> MSEKRSLPMVDVKIDDEDTPQLEKKIKRQSIDHGVGSEPVSTIEIIPSDSFRKYNSQGFKAKDTDLMGTQLESTFEQELSQMEHDMADQEEHDLSSFERKKLPTDFDPSLYDISFQQIDAEQSVLNGIKDENTSTVVRFFGVTSEGHSVLCNVTGFKNYLYVPAPNSSDANDQEQINKFVHYLNETFDHAIDSIEVVSKQSIWGYSGDTKLPFWKIYVTYPHMVNKLRTAFERGHLSFNSWFSNGTTTYDNIAYTLRLMVDCGIVGMSWITLPKGKYSMIEPNNRVSSCQLEVSINYRNLIAHPAEGDWSHTAPLRIMSFSISCAGRIGVFPEPEYDPVIQIANVVSIAGAKKPFIRNVFTLNTCSPITGSMIFSHATEEEMLSNWRNFIIKVDPDVIIGYNTTNFDIPYLLNRAKALKVNDFPYFGRLKTVKQEIKESVFSSKAYGTRETKNVNIDGRLQLDLLQFIQREYKLRSYTLNAVSAHFLGEQKEDVHYSIISDLQNGDSETRRRLAVYCLKDAYLPLRLMEKLMALVNYTEMARVTGVPFSYLLARGQQIKVVSQLFRKCLEIDTVIPNMQSQASDDQYEGATVIEPIRGYYDVPIATLDFNSLYPSIMMAHNLCYTTLCNKATVERLNLKIDEDYVITPNGDYFVTTKRRRGILPIILDELISARKRAKKDLRDEKDPFKRDVLNGRQLALKISANSVYGFTGATVGKLPCLAISSSVTAYGRTMILKTKTAVQEKYCIKNGYKHDAVVVYGDTDSVMVKFGTTDLKEAMDLGTEAAKYVSTLFKHPINLEFEKAYFPYLLINKKRYAGLFWTNPDKFDKLDQKGLASVRRDSCSLVSIVMNKVLKKILIERNVDGALAFVRETINDILHNRVDISKLIISKTLAPNYTNPQPHAVLAERMKRREGVGPNVGDRVDYVIIGGNDKLYNRAEDPLFVLENNIQVDSRYYLTNQLQNPIISI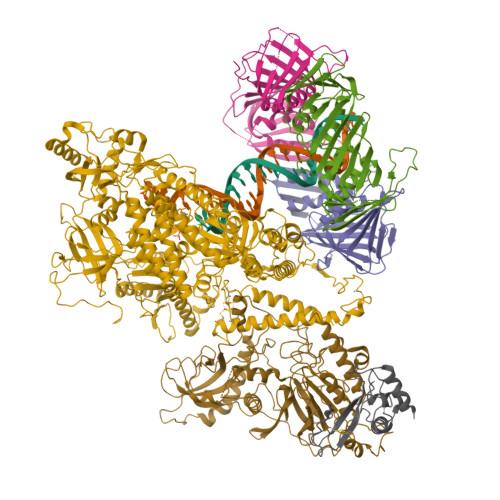VAPIIGDKQANGMFVVKSIKINTGSQKGGLMSFIKKVEACKSCKGPLRKGEGPLCSNCLARSGELYIKALYDVRDLEEKYSRLWTQCQRCAGNLHSEVLCSNKNCDIFYMRVKVKKELQEKVEQLSKW;> MDALLTKFNEDRSLQDENLSQPRTRVRIVDDNLYNKSNPFQLCYKKRDYGSQYYHIYQYRLKTFRERVLKECDKRWDAGFTLNGQLVLKKDKVLDIQGNQPCWCVGSIYCEMKYKPNVLDEVINDTYGAPDLTKSYTDKEGGSDEIMLEDESGRVLLVGDFIRSTPFITGVVVGILGMEAEAGTFQVLDICYPTPLPQNPFPAPIATCPTRGKIALVSGLNLNNTSPDRLLRLEILREFLMGRINNKIDDISLIGRLLICGNSVDFDIKSVNKDELMISLTEFSKFLHNILPSISVDIMPGTNDPSDKSLPQQPFHKSLFDKSLESYFNGSNKEILNLVTNPYEFSYNGVDVLAVSGKNINDICKYVIPSNDNGESENKVEEGESNDFKDDIEHRLDLMECTMKWQNIAPTAPDTLWCYPYTDKDPFVLDKWPHVYIVANQPYFGTRVVEIGGKNIKIISVPEFSSTGMIILLDLETLEAETVKIDI;> MDQKASYFINEKLFTEVKPVLFTDLIHHLKIGPSMAKKLMFDYYKQTTNAKYNCVVICCYKDQTIKIIHDLSNIPQQDSIIDCFIYAFNPMDSFIPYYDIIDQKDCLTIKNSYELKVSESSKIIERTKTLEEKSKPLVRPTARSKTTPEETTGRKSKSKDMGLRSTALLAKMKKDRDDKETSRQNELRKRKEENLQKINKQNPEREAQMKELNNLFVEDDLDTEEVNGGSKPNSPKETDSNDKDKNNDDLEDLLETTAEDSLMDVPKIQQTKPSETEHSKEPKSEEEPSSFIDEDGYIVTKRPATSTPPRKPSPVVKRALSSSKKQETPSSNKRLKKQGTLESFFKRKAK;>MLEAKFEEASLFKRIIDGFKDCVQLVNFQCKEDGIIAQAVDDSRVLLVSLEIGVEAFQEYRCDHPVTLGMDLTSLSKILRCGNNTDTLTLIADNTPDSIILLFEDTKKDRIAEYSLKLMDIDADFLKIEELQYDSTLSLPSSEFSKIVRDLSQLSDSINIMITKETIKFVADGDIGSGSVIIKPFVDMEHPETSIKLEMDQPVDLTFGAKYLLDIIKGSSLSDRVGIRLSSEAPALFQFDLKSGFLQFFLAPKFNDEE[3x]> REFTIDFSTQQSYVSSLNSIRTEISTPLEHISQGTTSVSVINHTPPGSYFAVDIRGLDVYQARFDHLRLIIEQNNLYVAGFVNTATNTFYRFSDFTHISVPGVTTVSMTTDSSYTTLQRVAALERSGMQISRHSLVSSYLALMEFSGNTMTRDASRAVLRFVTVTAEALRFRQIQREFRQALSETAPVYTMTPGDVDLTLNWGRISNVLPEYRGEDGVRVGRISFNNISAILGTVAVILNCHHQGARSVRAVNEESQPECQITGDRPVIKINNTLWESNTAAAFLNRKSQFLYTTGK;>[5x]ADCAKGKIEFSKYNEDDTFTVKVDGKEYWTSRWNLQPLLQSAQLTGMTVTIKSSTCESGSGFAEVQFNND;> MAMMXRRRRAX

Shiga toxin (Stx) is a major virulence factor of enterohemorrhagic Escherichia coli, which causes bloody diarrhea, hemorrhagic colitis, and sometimes fatal systemic complications, such as acute encephalopathy and hemolytic-uremic syndrome. Stx consists of a catalytic A-subunit and a B-subunit pentamer. The catalytic A-subunit is an RNA N-glycosidase that cleaves a specific adenine from 28S ribosomal RNA to inhibit eukaryotic protein synthesis. The B-subunit pentamer is responsible for high-affinity binding of Stx to the functional cell surface receptor, Gb3 (Galα[1–4]-Galβ[1–4]-Glcβ-ceramide).

Unexpectedly, a monomeric peptide with the same motif, Met-Ala-Met-Met-βAla-Arg-Arg-Arg-Arg-Ala (referred to as MMβA-mono), also inhibited the cytotoxicity of Stx1a and Stx2a with greater potency against Stx2a (relative IC50 = 59 and 9.6 µM, respectively). The binding site of MMβA-mono to the A-subunit was determined by X-ray crystallography using a co-crystal of MMβA-mono and the Stx2a holotoxin, which is a subtype that is most closely associated with the severity of the infection. The co-crystal was obtained by the soaking method. Diffraction to 1.6 Å-resolution showed that MMβA-mono was bound tightly to the catalytic A-subunit through electrostatic interactions of the Arg-cluster with Asp94 and Glu167 of the A-subunit and with Asp70 of the B-subunit, residues that are all present in the catalytic cavity. MMβA-mono occupied a wide region of the cavity, including Tyr77, Val78, Asp94, Ser112, Tyr114, Thr115, Glu167, Thr199, and Asp70. Also, Glu167 and Arg170, both of which are known to be essential for catalytic activity, were found to interact with Arg at position 8 of MMβA-mono. The replacement of each Arg of MMβA-mono with Ala resulted in a marked reduction in A-subunit binding. Replacement of both Arg residues with Ala at positions 8 and 9 abolished binding, indicating that these two Args are synergistically involved in the binding. The C-terminal Ala of MMβA-mono is present in the bottom of the catalytic pocket of the A-subunit; therefore, MMβA-tet cannot bind to the A-subunit because each C-terminal Ala of the motif (Met-Ala-Met-Met-βAla-Arg-Arg-Arg-Arg-Ala-) is connected to the core structure through a spacer. The structural information that defines the unique binding characteristics of MMβA-mono to Stx will be important in determining pharmacophores for the design of more precise and effective small-molecule inhibitors against Stxs.>[4x]S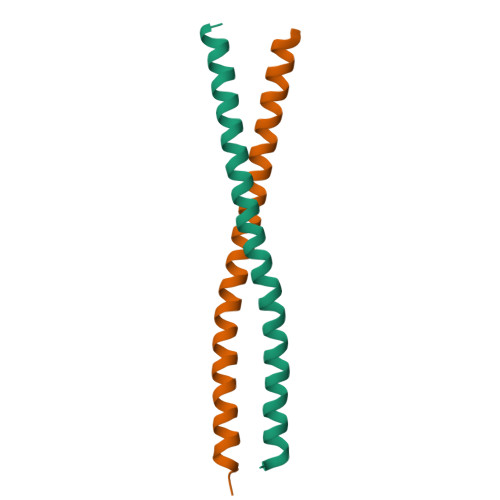LSSGTTEEELLRKLNEQRDILALMEVKMKEMKGSIRHLRLTEAKLREELREKDRLLAMAVIRKKHGM>[4x]MIISKEKTVSQEEMEELRLVARKTWRYFEDFVTEGQNYLPPDNFQEDPPNGVAERTSPTNIGLYLVSVIGARDLGYITTTEMVERIKKTLDTIEKMEKWNGHLYNWYNTKTLEPLRPYYVSTVDSGNLVGYLITVKEAIGEFLNKPLIDIELAKGLKDTIKMLNVKGITEDIFTTILSKTTLVPSEWEAFLNKIREKLLSSQDDLENIKRLKNIIIALKGEMKEFLVWTEFDESEKEQEIFKRYKEVFEEHSSPKELEKVYKNYLLEIEEVFKKATEEEKALLKSQKDKVAQALEKIKKLEAEIENIKSTIENLVEKTEFRHLYDEKRQLFSIGYNVEEEKLTKSYYDLLASEARQASFIAIAKKEVDKKHWFKLGRMLAIENRYKGLVSWSGTMFEYFMPLLVMRNYQNTLLDETYAFAVRVQKNYAKELGIPWGISESGFYAFDMNLNYQYKAFGVPSLGLKRGLSHDKVVAPYGSLLAIGVDVEGVLQNIRFFKKEGAEGKYGFYEAIDYTPERVPFGKKSAIVKSFMAHHQGMVFVALDNFINNNVMQKRFHKDPRIKAAQILLQEKMPMYLDITREEREGARKLEHHHHHH

Cyclic β-1,2-glucan synthase (CGS) is a key enzyme in production of cyclic β-1,2-glucans (CβGs) which are involved in bacterial infection or symbiosis to host organisms. BaCGS is composed of three regions responsible for the following steps: initiation (covalent bonding of glucose to CGS), elongation of linear β-1,2-glucan (LβGs) chains, adjustment of chain lengths of the glucans, and cyclization of the glucans by transglycosylation. Here we performed functional and structural analyses of the cyclization domain of CGS alone from Thermoanaerobacter italicus (TiCGSCy). In the present study, we explicitly showed that TiCGSCy domain alone produced CβGs by transglycosylation reaction without hydrolysis.

A ligand-free structure of TiCGSCy was determined at 3.9 Å resolution. An asymmetric unit contains almost identical four molecules (RMSD, 0.3 Å). The enzyme consists of a single (α/α)6-barrel domain with several inserted α-helices. Structure-based multiple amino acid alignment suggests that the additional α-helices in the middle region is unique to CGSs, and they are not found in SGLs. A large pocket observed in (α/α)6-barrel domain is expected to be a substrate binding site of TiCGSCy. The shape of the substrate pocket of TiCGSCy is similar to those of TfSGL and CpSGL in that the substrates observed in TfSGL and CpSGL complex structures can be potentially accommodated in the pocket, although the superimposed glucose moiety at subsite − 3 is a little too close to TiCGSCy. There is a sufficient space beyond 2-hydroxy group of the potential subsite − 4, which is consistent with the fact that TiCGSCy prefers Sopns with larger DPs. Contrarily, W1394 is likely to block binding of glucose moieties beyond subsite + 3. Taking into account the result of action pattern analysis that subsite + 4 should be occupied, side chain of W1394 may flip to make room for substrate binding. In the case of TiCGSCy, E1442 is found with a clear electron density at the position corresponding to that of the nucleophilic water in TfSGL, which attacks the anomeric carbon of the glucose moiety at subsite − 1.>MRLARFDGGRLGVVIGDEIADITALTGADPAQWPDMNMIRLIRDFEGLRGAIEAALPGLARIPLAQVSLETPVPWPNKIIAYPVNYHAHGREMQAQYRATNQGFFLKPGSALSGPTDPVVLPAVPGREVHHE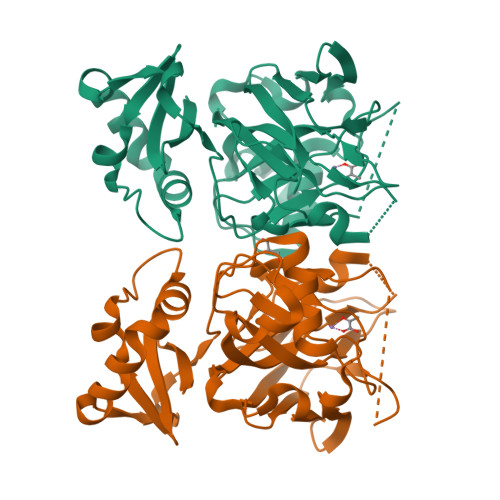SELAIIIGKTCRSVAREDWKDVVFGYACLLDMVVRGREERVFRKAYDTFCPVGPWITTADAVNDPATLDMKLWVNDDLRQKANTRDLVLDIPGMIATASAVMTLQPGDIIATGTPEGVGPVVDGDRIRIVIDQVGEMAVDVVQGQEGMTEVFAQPYVPPIIKQALEHHHHHH[2x]>[2x]MTSDTKPQAKDLTHLLSNESKARQTSPLKGIFKYYKQPGITFLGGGLPLSDYFPFEKVTADIPTPSFSGGIGAPIEGENKTTIEVFKKAADNVPDQIELARSLQYGSTFGLPEFLQFIKEHTDMVHKVPYENWDVIVSVGNTEAWDSTLRTFCSKGDTILVEEYTFSSALESANGQGVNTVPVTMDEFGIIPEKLEELMSRWVGNKPKFLYTICTGQNPTGSSL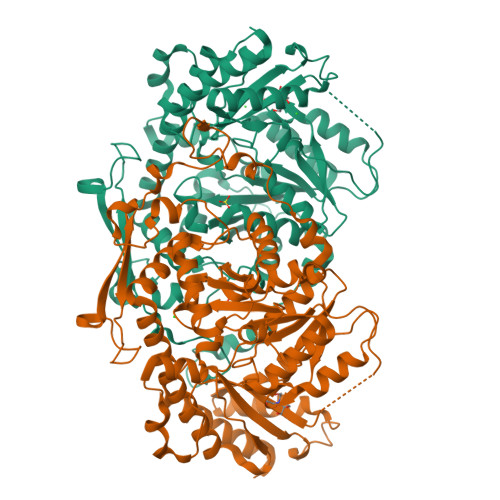SAERRKQIYDIACKYDFLIIEDEPYYFLQMETYTKDKAAREGKAVHDHDEFLKALVPSFISLDVEGRVVRLDSFSKVLAPGLRLGWIVGQKDLLERYVRLHEVSVQNPSGFSEALANALLRKWGHSGYLDWLIGLRAEYTHKRDVAIDALDQFVPKEVSSFNPPVAGMFFTVTLDASKHPKYKEFLEDPLKVEAAVHEQAIKQGCLLAPGSWFKAEGQSSPPQKNLPANPSHKTHIFFRGTYAAVPLDQLVVGLEKFGKAVRAEFGL>MWSHPQFEKSAMPFVGGAESGDPLGAGRPIGDDECEQYTSSVSLARMLYGGDLAEWVPRVHPKTTIERQQHGPVTFPNASAPTARCVTVVRAPMGSGKTTALIRWLREAIHSPDTSVLVVSCRRSFTQTLATRFAESGLVDFVTYFSSTNYIMNDRPFHRLIVQVESLHRVGPNLLNNYDVLVLDEVMSTLGQLYSPTMQQLGRVDALMLRLLRTCPRIIAMDATANAQLVDFLCGLRGEKNVHVVVGEYAMPGFSARRCLFLPRLGTELLQAALRPPGPPSGPSPDASPDARGATFFGELEARLGGGDNICIFSSTVSFAEIVARFCRQFTDRVLLLHSLTPLGDVTTWGQYRVVIYTTVVTVGLSFDPLHFDGMFAYVKPMNYGPDMVSVYQSLGRVRTLRKGELLIYMDGSGARSEPVFTPMLLNHVVSSCGQWPAQFSQVTNLLCRRFKGRCDASACDTSLGRGSRIYNKFRYKHYFERCTLACLSDSLNILHMLLTLNCIRVRFWGHDDTLTPKDFCLFLRGVHFDA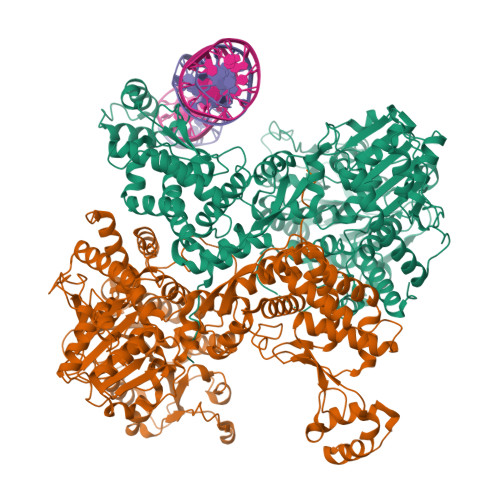LRAQRDLRELRCRDPEASLPAQAAETEEVGLFVEKYLRSDVAPAEIVALMRNLNSLMGRTRFIYLALLEACLRVPMATRSSAIFRRIYDHYATGVIPTINVTGELELVALPPTLNVTPVWELLCLCSTMAARLHWDSAAGGSGRTFGPDDVLDLLTPHYDRYMQLVFELGHCNVTDGLLLSEEAVKRVADALSGCPPRGSVSETDHAVALFKIIWGELFGVQMAKSTQTFPGAGRVKNLTKQTIVGLLDAHHIDHSACRTHRQLYALLMAHKREFAGARFKLRVPAWGRCLRTHSSSANPNADIILEAALSELPTEAWPMMQGAVNFSTL[2x]>GAGTTTTSVTVHKLLATDGDMDKIANELETGNYAGNKVGVLPANAKEIAGVMFVWTNTNNEIIDENGQTLGVNIDPQTFKLSGAMPATAMKKLTEAEGAKFNTANLPAAKYKIYEIHSLSTYVGEDGATLTGSKAVPIEIELPLNDVV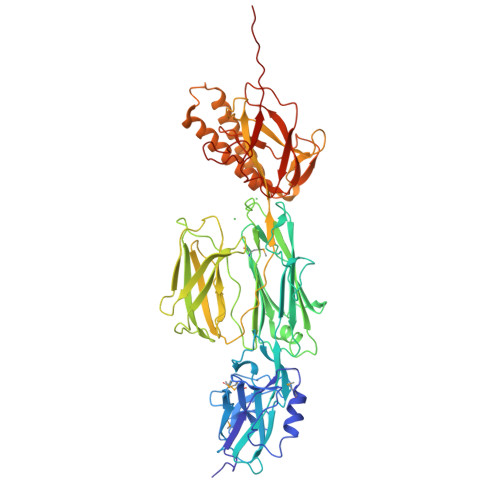DAHVYPKNTEAKPKIDKDFKGKANPDTPRVDKDTPVNHQVGDVVEYEIVTKIPALANYATANWSDRMTEGLAFNKGTVKVTVDDVALEAGDYALTEVATGFDLKLTDAGLAKVNDQNAEKTVKITYSATLNDKAIVEVPESNDVTFNYGNNPDHGNTPKPNKPNENGDLTLTKTWVDATGAPIPAGAEATFDLVNAQTGKVVQTVTLTTDKNTVTVNGLDKNTEYKFVERSIKGYSADYQEITTAGEIAVKNWKDENPKPLDPTEPKVVTYGKKFVKVNDKDNRLAGAEFVIANADNAGQYLARKADKVSQEEKQLVVTTKDALDRAVAAYNALTAQQQTQQEKEKVDKAQAAYNAAVIAANNAFEWVADKDNENVVKLVSDAQGRFEITGLLAGTYYLEETKQPAGYALLTSRQKFEVTATSYSATGQGIEYTAGSGKDDATKVVNKKITIPQTGG[3x]>MERPQLDSMSQDLSEALKEATKEVHIRAENSEFMRNFQKGQVSREGFKLVMASLYHIYTALEEEIERNKQNPVYAPLYFPEELHRRAALEQDMAFWYGPHWQEAIPYTPATQHYVKRLHEVGGTHPELLVAHAYTRYLGDLSGGQVLKKIAQKAMALPSSGEGL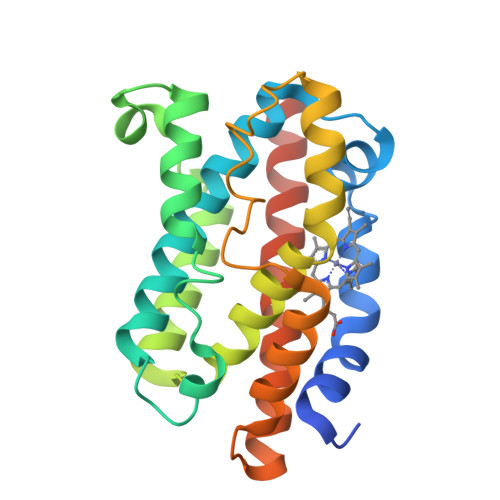AFFTFPSIDNPTKFKQLYRARMNTLEMTPEVKHRVTEEAKTAFLLNIELFEELQALLTEEHKDQSPSQ[7x]> MNINLTLIGQAIAFAFFVAFCMKFVWPPLINAISERQRKIADGLNAAEKAKADLADAQAQVKQELDAAKAQAAQLIEQANRRAAQLIEEARTQAAAEGE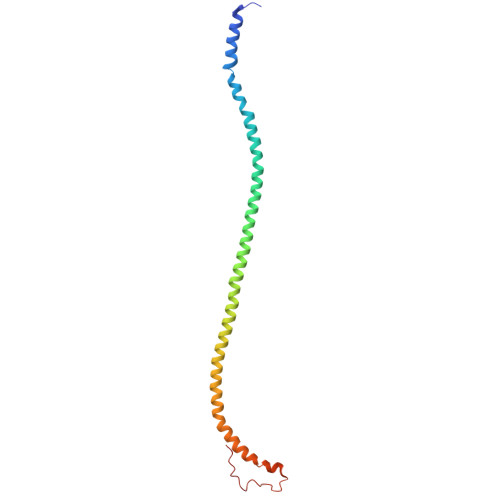RIRQQAKEAVDQEINSAREELRQQVAALAVTGAEKILNQQVDAEAHNAMLSQLAAKL>[3x]GSRMSGNNMSTPLPAIVPAARKATAAVIFLHGLGDTGHGWAEAFAGIRSSHIKYICPHAPVRPVTLNMNVAMPSWFDIIGLSPDSQEDESGIKQAAENIKALIDQEVKNGIPSNRIILGGFSQGGALSLYTALTTQQKLAGVTALSCWLPLRASFPQGPIGGANRDISILQCHGDCDPLVPL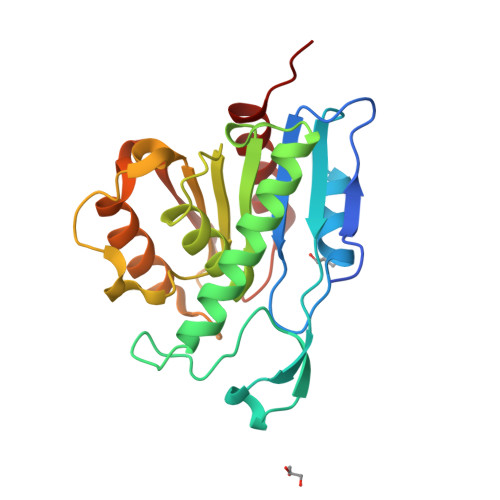MFGSLTVEKLKTLVNPANVTFKTYEGMMHSSCQQEMMDVKQFIDKLLPPID;> GSRMSGNNMSTPLPAIVPAARKATAAVIFLHGLGDTGHGWAEAFAGIRSSHIKYICPHAPVRPVTLNMNVAMPSWFDIIGLSPDSQEDESGIKQAAENIKALIDQEVKNGIPSNRIILGGFSQGGALSLYTALTTQQKLAGVTALSCWLPLRASFPQGPIGGANRDISILQCHGDCDPLVPLMFGSLTVEKLKTLVNPANVTFKTYEGMMHSSCQQEMMDVKQFIDKLLPPIDA Tubulin-binding cofactor A (TBCA) participates in microtubule formation, a key process in eukaryotic biology to create the cytoskeleton. Tubulin-binding cofactor (TBC) proteins, of which there are at least five, are intimately involved in this assembly process, but the details about specific contributions are limited. In order to underpin dissection of TBC function and delineation of structure–activity relationships, we have instigated studies of the trypanosomatid proteins and now report a crystallographic study of one, TBCA, from Leishmania major. This protein is thought to make an early contribution to the assembly process through delivery of β-tubulin onto a second protein, TBCD. In one model for microtubule biogenesis this TBCD–β-tubulin complex then facilitates α/β-tubulin heterodimer formation.

The structure of LmTBCA was determined by the SAD approach and was refined to 1.9 Å resolution. There was no reliable electron density for the first 18 residues and the model comprises residues Glu19–Ser125. The protein fold consists of three α-helices (α1–α3) aligned in an antiparallel fashion. Helices α1 and α2, each comprising ten helical turns, are distorted, with bends of approximately 20–25°, giving the molecule an overall curved appearance. The proline at position 80 in LmTBCA is strictly conserved in these structures and appears to contribute to a bend in α2 in all cases, although the effect appears most pronounced in the Leishmania protein. Although LmTBCA did display a dimeric assembly, it is distinct from that observed for ScRbl2p and is driven by the formation of a disulfide linkage. However, the formation of this Cys58–Cys58 disulfide bond may have stabilized the structure of the α1–α2 loop, and as Cys58 is not a conserved residue in TBCA sequences, it may have fortuitously aided in the crystallization of LmTBCA. We do not ascribe any biological significance to the observation of a covalent dimer of LmTBCA formed owing to a disulfide linkage. The concave surface of LmTBCA might therefore present a favourable site for interaction, driven by electrostatic attraction, with β-tubulin. The presence of a localized region enriched in basic residues, which are conserved in TBCA from evolutionarily diverse species, together with the overall acidic properties of the C-terminal tails of β-tubulins, hints that electrostatic forces might be relevant for complex formation, but further work is required to address such a hypothesis.

> GHMSDSTESTNRFASNVRQAEAPNEKTLRIKVSALKRTIKDLEFAKREVERELQRLDTLCQSDPDRVPQQTKVVDEAQMMVPHSVNRIMASVKDLSDYLEKEGSTVSNEELLDLARATMADGQAAVS> KMLEEIMKYEASILTHDSSIRYLQEIYNSNNQKIVNLKEKVAQLEAQCQEPCKDTVQIHDITGKDCQDIANKGAKQSGLYFIKPLKANQQFLVYCEIDGSGNGWTVFQKRLDGSVDFKKNWIQYKEGFGHLSPTGTTEFWLGNEKIHLISTQSAIPYALRVELEDWNGRTSTADYAMFKVGPEADKYRLTYAYFAGGDAGDAFDGFDFGDDPSDKFFTSHNGMQFSTWDNDNDKF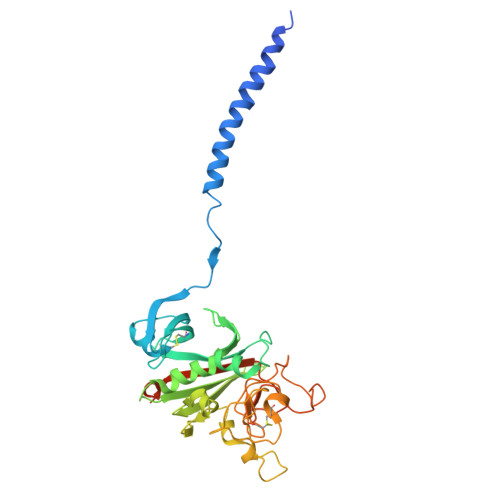EGNCAEQDGSGWWMNKCHAGHLNGVYYQGGTYSKASTPNGYDNGIIWATWKTRWYSMKKTTMKIIPFNRLTIGEGQQHHLGGAKQAGDV>VDSVYRTRSLGVAAEGIPDQYADGEAARVWQLYIGDTRSRTAEYKAWLLGLLRQHGCHRVLDVACGTGVDSIMLVEEGFSVTSVDASDKMLKYALKERWNRRKEPAFDKWVIEEANWLTLDKDVPAGDGFDAVICLGNSFAHL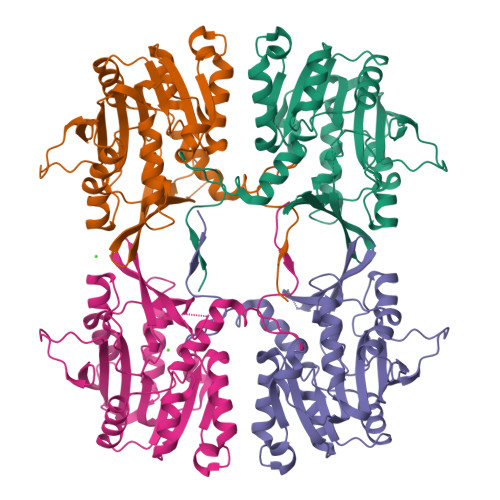PDSKGDQSEHRLALKNIASMVRPGGLLVIDHRNYDYILSTGCAPPGKNIYYKSDLTKDITTSVLTVNNKAHMVTLDYTVQVPGAGRDGAPGFSKFRLSYYPHCLASFTELVQEAFGGRCQHSVLGDFKPYRPGQAYVPCYFIHVLKKTG[4x]> AQIGPVTDLHITNANISPDGFSRPAVLAGGTFPGPTIAGNTGDNFQITVFNDLTDPSMLTDTSIHWHGLFQKGTNWADGPAFVTQCPIITGQSFDYNFNVPGQAGTFWYHSH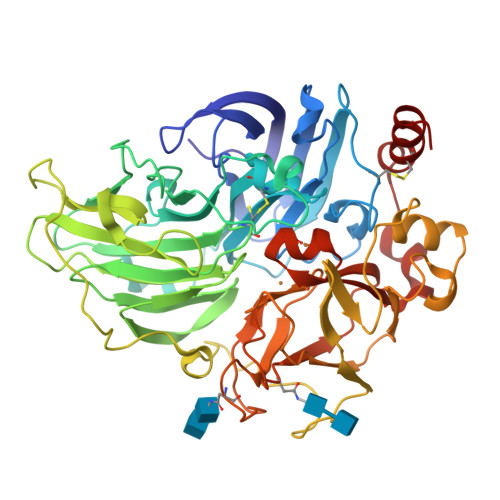LSTQYCDGLRGPFVVYDPNDPNASLYDVDDDTTIITLADWYHTLAQQEPIGAAITADATLINGLGRSFTNTTASPLSVITVQSGKRYRMRLVSISCDPNYLFSIDGHDMTIIEVDGVNSQQLTVDQIQIFAAQRYSFVLNANQPVGNYWIRAQPNSGGQGFDGGINSAILRYEGATVEDPTTTAPTTFSNPLVETDLHPLADLGVPGQPFRGGADDPLVLNLAFANGRFSIDGVSFVPPTVPVLLQILSGAQNAQDLLPAGSVISLPSNSVIEVALPAGAAGGPHPFHLHGHNFAVVQSANNATPNYVNPIWRDTVSIGGTGDNVTIRFTTNNPGPWFLHCHIDWHLEAGFAIVFAEDIPDTASANPVPQAWSDLCPAYDQAHNIS> GAMGSEKSPSAQELKEQGNRLFVGRKYPEAAACYGRAITRNPLVAVYYTNRALCYLKMQQHEQALADCRRALELDGQSVKAHFFLGQCQLEMESYDEAIANLQRAYSLAKEQRLNFGDDIPSALRIAKKKRWNS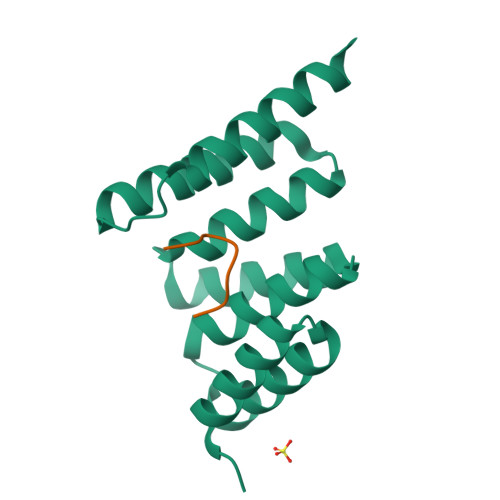IEERR;> GPTIEEVD> MHHHHHHMVKGHTTGLSLNNDRLYKLTYSTEVLLDRGKGKLQDSVGYRISSNVDVALLWRNPDGDDDQLIQITMKDVNVENVNQQRGEKSIFKGKSPSKIMGKENLEALQRPTLLHLIHGKVKEFYSYQNEAVAIENIKRGLASLFQTQLSSGTTNEVDISGNCKVTYQAHQDKVIKIKALDSCKIARSGFTTPNQVLGVSSKATSVTTYKIEDSFVIAVLAEETHNFGLNFLQTIKGKIVSKQKLELKTTEAGPRLMSGKQAAAIIKAVDSKYTAIPIVGQVFQSHCKGCPSLSELWRSTRKYLQPDNLSKAEAVRNFLAFIQHLRTAKKEEILQILKMENKEVLPQLVDAVTSAQTSDSLEAILDFLDFKSDSSIILQERFLYACGFASHPNEELLRALISKFKGSIGSSDIRETVMIITGTLVRKLCQNEGCKLKAVVEAKKLILGGLEKAEKKEDTRMYLLALKNALLPEGIPSLLKYAEAGEGPISHLATTALQRYDLPFITDEVKKTLNRIYHQNRKVHEKTVRTAAAAIILNNNPSYMDVKNILLSIGELPQEMNKYMLAIVQDILRFEMPASKIVRRVLKEMVAHNYDRFSRSGSSSAYTGYIERSPRSASTYSLDILYSGSGILRRSNLNIFQYIGKAGLHGSQVVIEAQGLEALIAATPDEGEENLDSYAGMSAILFDVQLRPVTFFNGYSDLMSKMLSASGDPISVVKGLILLIDHSQELQLQSGLKANIEVQGGLAIDISGAMEFSLWYRESKTRVKNRVTVVITTDITVDSSFVKAGLETSTETEAGLEFIST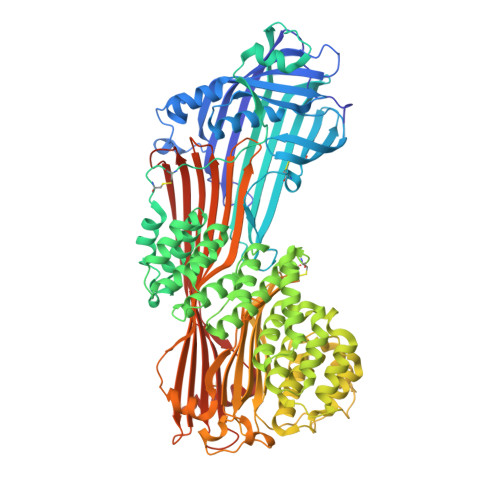VQFSQYPFLVCMQMDKDEAPFRQFEKKYERLSTGRGYVSQKRKESVLAGCEFPLHQENSEMCKVVFAPQPDSTSSGWF> HDTLLILGDSLSA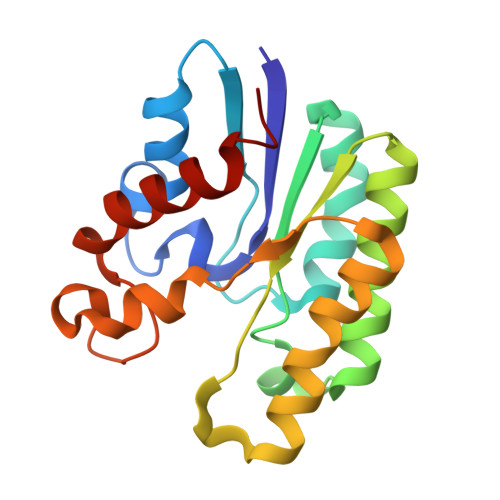GYRMSASAAWPALLNDKWQSKTSVVNASISGDTSQQGLARLPALLKQHQPRWVLVELGGNDGLRGFQPQQTEQTLRQILQDVKAANAEPLLMQIRLPANYGRRYNEAFSAIYPKLAKEFDVPLLPFFMDEVGLKPQWMQDDGIHPNRDAQPFIADWMAKQLQPLVN> KSSKALNEAAEQGDLAKVKNLVQKNKIDLNAQDETGMTPLMNAAMGGNLDIVKFLLSKKVNLEL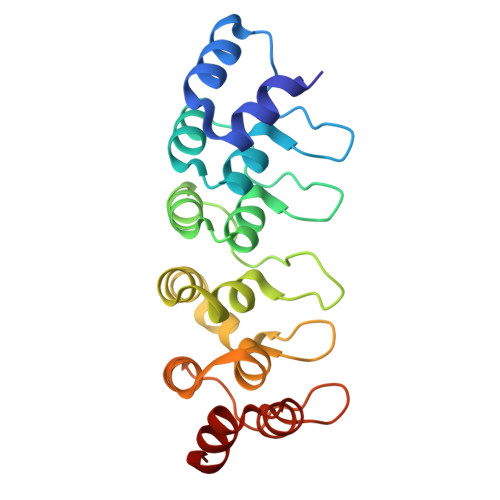KNNGGETALAFAVTNDAYDVAEELIKAGANVDIIVAGDEGDTLFMRAAQNNKKTAESILAKNKSLINKANTLGETALFAVARYGTPADIDFLIKKGADLKLKNKKGQTALDVAKEASNQDTAKALSKKK>MSKIVKIIGREIIDSRGNPTVEAEVHLEGGFVGMAAAPSGASTGSREALELRDGDKSRFLGKGVTKAVAAVNGPIAQALIGKDAKDQAGIDKIMIDLDGTENKSKFGANAILAVSLANAKAAAAAKGMPLYEHIAELNGTPGKYSMPVPMMNIINGGEHADNNVDIQEFMIQPVGAKTVKEAIRMGSEVFHHLAKVLKAKGMNTAVGDEGGYAPNLGSNAEALAVIAEAVKAAGYELGKDITLAMDCAASEFYKDGKYVLAGEGNKAFTSEEFTHFLEELTKQYPIVSIEDGLDESDWDGFAYQTKVLGDKIQLVGDDLFVTNTKILKEGIEKGIANSILIKFNQIGSLTETLAAIKMAKDAGYTAVISHRSGETEDATIADLAVGTAAGQIKTGSMSRSDRVAKYNQLIRIEEALGEKAPYNGRKEIKGQA[4x];> RRYRDERYPTQSPMPLTVACASPELASGKVWIRYPI;> RDERYPTQSPMPLTVACASPELASGKVWIRYPIVR

For E. coli, the key enzyme of RNA metabolism and riboregulation is RNase E, a conserved endoribonuclease which forms a large multi-enzyme complex, known as the degradosome, that incorporates the DEAD-box helicase RhlB, the phosphorylytic exoribonuclease polynucleotide phosphorylase (PNPase) and the glycolytic enzyme enolase. The C-terminal half of the enzyme, which is considerably more variable in molecular evolution compared to the N-terminal half, provides the scaffold of the degradosome assembly. This scaffolding region is predicted to be predominantly natively disordered, with small linear recognition motifs that interact with the canonical protein components, RNA and the cytoplasmic membrane that consequently compartmentalizes the assembly to the periphery of the cytoplasm. A segment of the E. coli RNase E C-terminal domain, encompassing the binding sites for enolase and RhlB (corresponding to residues 603–850; hereafter RNase E 603–850), also bears two arginine-rich RNA binding domains, which are referred to as the RNA-binding domain (RBD) and AR2 (arginine-rich region 2).

To explore the structural impact of enolase binding on the adjacent AR2 element, the enzyme was co-crystallized in complex with the RNase E segment encompassing the EBS and AR2 regions. Well diffracting crystals were obtained and the structure solved and refined to 2.0 Å resolution. Two enolase dimers occupy the asymmetric unit. In agreement with earlier results, the segment with residues 822–849 interacts with the intra-protomer cleft of the enolase dimer. The cleft has 2-fold symmetry and the EBS can enter the cleft in one of two equivalent orientations. Notably, in one of the enolase dimers, the EBS is superimposed in those two orientations. Although some broken density could be seen for the N-terminal side of the EBS, no features could be resolved unambiguously for the AR2 segment in either of the enolase dimers of the asymmetric unit. Nonetheless, some portions of the AR2 peptide could be fitted to the density at low occupancy, but it is clear that this segment assumes multiple conformations. This suggests that the AR2 region possesses significant flexibility and does not adapt a single conformation when enolase is bound to the neighboring EBS.> MTALPPPPSANVAVSFTAAPAEPLSRGEVKAASLKLELQ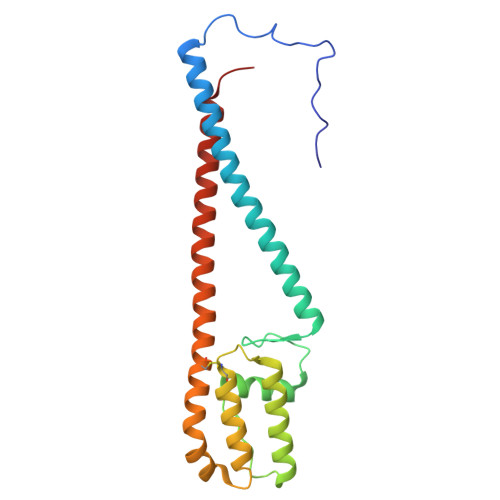NIERELKDWWMSRKILRDRNIGLFNLLQHHNFAGLSVNNAKLSDSQRVMWTDLVQGKPDVEDKLSVDAREMKVDMYEKLFKQAADLENPCRMPGVAYLRCLRDTLTETQSARRSSCLNAFSSFDACRTGLLKQQSAAVENSLVRQNMADVRAKALFERRAVLLDLVEGK>[4x]MRDVAIIGYGQTKFGELWEDSFRDLIVEAGVKAIKDANVDGGDIDAMYIGNMSGGLFVGQEHIASLIADHAGLNPVPCTRVEAACASGSLALRSAVLSVASGHHDVVLAGGVEKMTDVEDATAAIASASDQEWEAFFGATFPSLYAMMARRYMYQYGLTIEELSMWSVIAHENATKNKYAQFGFKTTLEQVMNASPVADPLTLMHCSPVSDGASALIVCDADKAE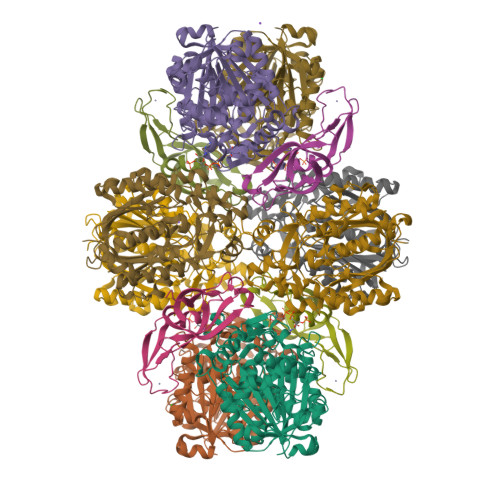EFAPKDEIIYIKASTQASDTIALHDREDMTTLNAAKVASEKAYKLAKIAPEKIDVAEVHDCFAINGLILVEDLGFCKKGDAGKVIDEGKIRIDYDDFVTVNPSGGLKAAGHALGATGIRQVGELYWQLKQDKECKDRQATIKNGYGIAANVGGTGGTVCVHLLSDKR;>MVVRSWRHMKERYNLIGTRCKTCGKVYFPSRTVCPDCRRKGELEEFQLSGKGKIYTYSIVYAPPKEFNKLTPYVIAIVELEEGPKVTAQVDCDINKISIGIPVEAAFRRIKEDGKDGIISYGYKFVPITE[4x];>[4x]MKDIGIVGYGSYIPKYRIKVEEIAKVWGKDPEAIKKGLVVNEKSVPSPDEDTATIAVEAARNAVKRAGINAEKIGAVYVGSESHPYAVKPTSATVAEAIGATPDLTAADLEFACKAGTAGIQMCMGLVGSGLIEYGMAIGADTAQGAPGDALEYTASAGGAAYIIGNKKDEMIAVFNGTYSYTTDTPDFWRREGQSYPKHGGRFTGEPAYFKHVLNAAKGIMEKMGTTVKDYDYCVFHQPNGKFYIKAAKSLGFTNEQYKYGLLTPYLGNTYSGAVPLGLSNILDHAEEGARILAVSYGSGAGSDAFDITVTERIKEVVDKAPKTLDLLNRKKYIDYAVYVKYRGKIKI> MSVDPMTYEAQFFGFTPQTCMLRIYIAFQDYLFEVMQAVEQVILKKLDGIPDCDISPVQIRKCTEKFLCFMKGHFDNLFSKMEQLFLQLILRIPSNILLPEDKCKETPYSEEDFQHLQKEIEQLQEKYKTELCTKQALLAELEEQKIVQAKLKQTLTFFDELH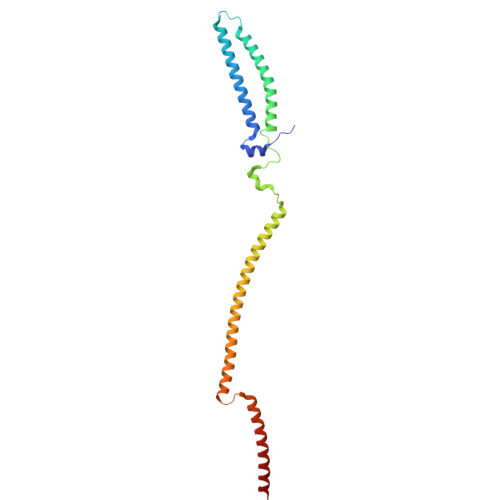NVGRDHGTSDFRESLVSLVQNSRKLQNIRDNVEKESKRLKIS> GCGTCA;>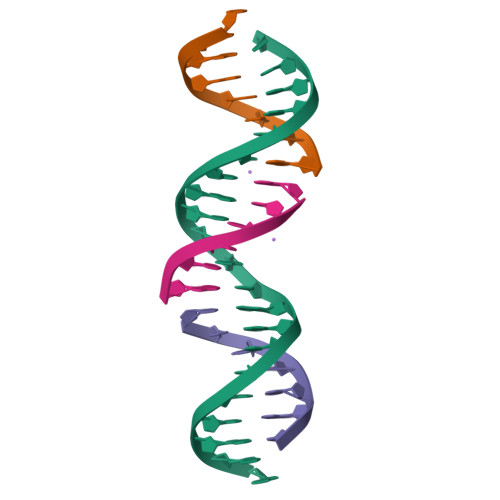 GAACGACAGTGACGCCGACTC;> TCGAGTCG;> CTGTCGT>[2x]DPWAMTAEEKAKAVPLIHQEGNRLYREGHVKEAAAKYYDAIACLKNLQMKEQPGSPEWIQLDQQITPL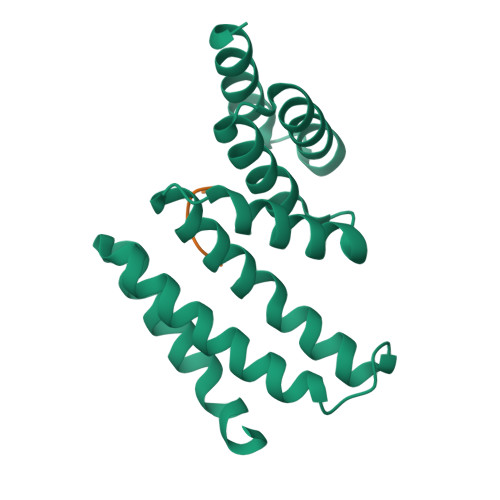LLNYCQCKLVVEEYYEVLDHCSSILNKYDDNVKAYFKRGKAHAAVWNAQEAQADFAKVLELDPALAPVVSRELQALEARIRQKDEEDKARFRGIFSH;>AEDDVE[2x]>MNSLLRLPALKRGVFTMSKRGLATTVSPKTRTSNLKNGLTIASESNPLVQTATVGVWIDAGSRNENAYNNGTAHFFEHLAFKGTDKRSQHQLELDIENMGGHLNAYTSRESTVYYAKSFKDDVPKSVEILADILQHSKLAESAIDREREVITRELEEVNKQYEEVVFDHLHATAFMNQPLGRTILGPRENIQTITNTELRKFITENYTADRMVLVGAGAVDHDALVELAEKYFSHLPSSQSPVPLGTPRSSGEDANQNPIPNFVGSEVRLRDDTMPVAHIAIAVEGVSWTSEDYYTALVAQAIIGNYDRAVGTSRHQGSRLSNIVSENNLANSFQSFSTSYSDTGLWGIYLTSENTTQIDDLVHFTLKEWNRLSTSVSNLQVERAKSQLKAGLLLSLDGTTYVAEDIGRQLTTLGRRVTPAEVEAKLEAVTEHDVRAWAQKTLYDKDIALVGLGPIEGLYDYNRIRNDMSMMRW[2x];>[2x]MTRGVPRLAVAARHFSTAEAAGVKVAAQDGQSPISDLSVVLRGGSRYATVPGVSHILEKFAFQNTVPKSALRFVRELELFGGKLYTHTTREHIVLRTQFLKQDLPYFVDAFANVLKETKFQQFELTERVAPVAELDLLKRESDPAFTALEAAHEVAFRTGLGNSVYAQGYSPVTLEDVKEFARQVYAKQNVAVVGNNVVPADLQQLVGTAFADLQEGSKVTQAGTTTLHGGEARVRTSTGNALTIALPIAEPKPVYHALASFLGGPASMPWSVGASPLAQATVGTHTSVKATYHNYGDAGLFAITIKGDSPAEISQVAHKAVQALKDTGAEVTEEQAARAYAKSKFAAAEAFENPDSSASVIGMELLSGVSRIAPENVQKFTPAELSEAAAQLSASAKPVVAAVGQVHALPFADELF;>MALRKKNSLLNMANSYVLDSPQPSNLNYFWNFGSLLALCLVIQLATGITLAMHYTSHASLAFDSVEHIMRDVNFGWFIRYAHANTASFFFICIYAHMGRNIYYGSYKTPRVLPWSIGVIIFLLLIITAFMGYVLVFGQMSLWGATVICNLVSAIPWLGEDIVHFLWGGFSVGNPTLQRFFALHYLMPFVLAVFALLHLIALHTAGSSNPLGITSNVDKLSMHPYYSFKDLITVFAFLLMFTLFVFFSPDKLGHPDNYIPANPMVTPASIVPEWYLLPFYAILRAIPDKLGGVIAMVAAILILLILPIVDRSIIRGNAFKPISKLLFGFFICNFLLLGVLGQVHIEPPFIVLGQICTIFYFSYFLILLPMVSTIENIFFYIGSLRK[2x];>[2x]MRRRRIGVWPENRRVSRLWVSLSPRSCVTCPVPTNQNPPINNHHTPILTQMFKAIPLRQALLGISSAVCAGATTTYYYTTKAEAMTAAEHGLHPAEYPWPQNGMLSTFDHASLRRGYQVYKEVCAACHSLDRIAWRNLVGVTHTTDEAKAFAEELEYDDEPDDEGNPRKRPGKLADYIPGPYPNEQAARAANQGALPPDLSLIAKARHGGADYIFALLTGYPDEPPAGVVLAPGMNYNPYFPGGGIGMARTLFDGVVEYEDGTPATTSQMAKDVAAFLTWAAEPEHDERKKLGLKAIIVISAMLGLSVYIKKFKWSPIKNRKFIYNPPKN;>MSLLRTAAQAVKAPKAYTPLVAAKAFAQTRSVSSQPIGGKSTYKIPDFTPYLKKDRNTDANRLFSYFMIGSFGMLSAAGAKATVQDFLSNMSASADVLAMAKVEVKLGAIPLGKNVIIKWRGKPIFIRHRTSEEIEEANEVNVATLRDPQTDDERVQKPEWLVMIGVCTHLGCVPIGEAGDFGGWFCPCHGSHYDISGRIRRGPAPLNLEIPEYDFADAETLVIG[2x];>MSYFLTLASEVAESLLPTVAFASEEEKEQDEPVEVESDDDESEEKEDDDEEEDEDDDDDDDDDEVPDPAIALHEAAAEGPCHDFKHHFDECVERVTKAQEAEDYDHAEYKEDCVEEFFHLQHCINDNTADKLFRVLK[2x];>[2x]MASITSVVKTSELILKSPLLSKIVVPLAKTYVKFSGYRQLGFKMNDLIIEETPNMQLALRRLPPTESYDRVYRLIRATQFSLSHKLATGNDITKPEEDDHYLIPYILDVEAEAFEKDALDNLEVVKRK;>MGGNG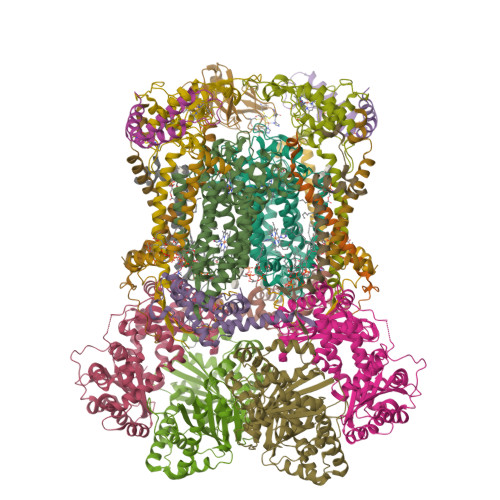HYMGWWGHMGSPPQKGIAGYTISPFAARPFAGVVHAAIFNTFRRTKNQALFVILPVSFFYYVWTQASEKNEWLYTKAGRHELAKALAE[2x];>[2x]MAWATTFYNVFVKRNSAFVATILASAFVFDMTFETAIDNFWDRINAGKQWKDIRHKYIEAAGDDDEDD;>MICGEGDYVKKPSYKIVPHFLGFNIPTVSKWIPIFGIWGAAAGIGALFLIEGVPRTRQDILSKIPIIGEHWIREIPASDNPF[2x]> IIGGRESRPHSRPYMAYLQIQSPAGQSRCGGFLVREDFVLTAAHCWGSNINVTLGAHNIQRRENTQQHITARRAIRHPQYNQRTIQN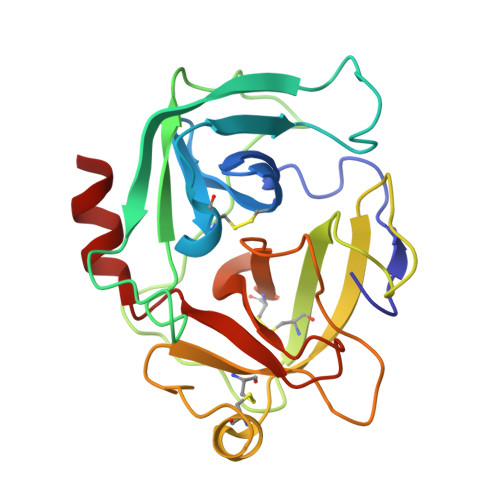DIMLLQLSRRVRRNRNVNPVALPRAQEGLRPGTLCTVAGWGRVSMRRGTDTLREVQLRVQRDRQCLRIFGSYDPRRQICVGDRRERKAAFKGDSGGPLLCNNVAHGIVSYGKSSGVPPEVFTRVSSFLPWIRTTMR> DLYFNPRFLADDPQAVADLSRFENGQELPPGTYRVDIYLNNGYMATRDVTFNTGDSEQGIVPCLTRAQLASMGLNTASVAGMNLLADDACVPLTTMVQDATAHLDVGQQRLNLTIPQAFMSNRARGYIPPELWDPGINAGLLNYNFSGNSVQNRIGGNSHYAYLNLQSGLNIGAWRLRDNTTWSYNSSDRSSGSKNKWQHINTWLERDIIPLRSRLTLGDGYTQGDIFDGINFRGAQLASDDNMLPDSQRGFAPVIHGIARGTAQVTIKQNGYDIYNSTVPPGPFTINDIYAAGNSGDLQVTIKEADGSTQIFTVPYSSVPLLQREGHTRYSITAGEYRSGNAQQEKPRFFQSTLLHGLPAGWTIYGGTQLADRYRAFNFGIGKNMGAL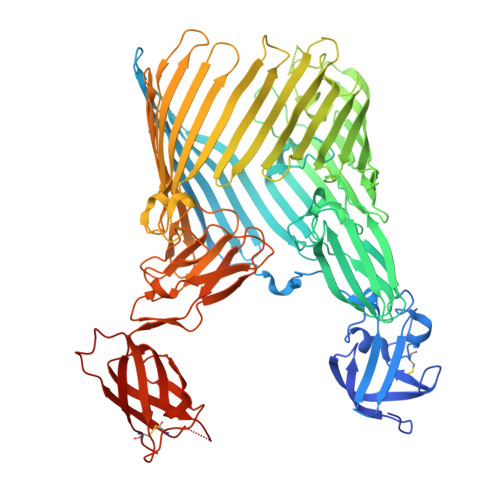GALSVDMTQANSTLPDDSQHDGQSVRFLYNKSLNESGTNIQLVGYRYSTSGYFNFADTTYSRMNGYNIETQDGVIQVKPKFTDYYNLAYNKRGKLQLTVTQQLGRTSTLYLSGSHQTYWGTSNVDEQFQAGLNTAFEDINWTLSYSLTKNAWQKGRDQMLALNVNIPFSHWLRSDSKSQWRHASASYSMSHDLNGRMTNLAGVYGTLLEDNNLSYSVQTGYAGGGDGNSGSTGYATLNYRGGYGNANIGYSHSDDIKQLYYGVSGGVLAHANGVTLGQPLNDTVVLVKAPGAKDAKVENQTGVRTDWRGYAVLPYATEYRENRVALDTNTLADNVDLDNAVANVVPTRGAIVRAEFKARVGIKLLMTLTHNNKPLPFGAMVTSESSQSSGIVADNGQVYLSGMPLAGKVQVKWGEEENAHCVANYQLPPESQQQLLTQLSAECRSAWSHPQFEK> MDSASKEETLEKLDQEITVN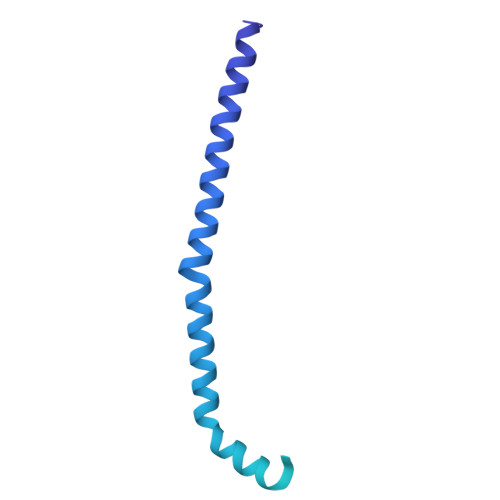LQKIDSNLSFCFHKITQDIIPHVATYSEICERIMDSTEWLGTMFQETGLVNLQANAAAPVGNAPVKSLVSNNVGIFPTSAEEASRQSQTDNGPNEADSAVHVNRDVHSMFNNDSIDDFHTANITSTGQILKLPDSSDEDTGSEAVPSREQTDLTGEGHGGADDEQDESTIQRQSRKRKISLLLQQQYGSSSSMVPSPIVPNKMRKQLAHEEHINNDGDNDDENSNNIESSPLKQGHHHPKGQADDNNEGPDEEESTKEVPKPGTIIHFSTNR>[2x]MTVPIAIIGTGIAGLSAAQALTSAGHQVH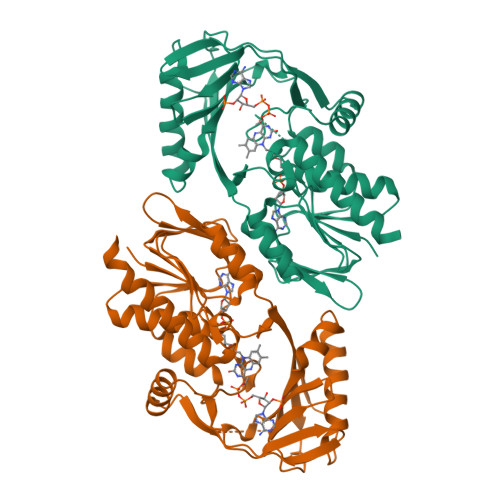LFDKSRGSGGRMSSKRSDAGSLDMGAQYFTARDRRFATAVKQWQAQGHVSEWTPLLYNFHGGRLSPSPDEQVRWVGEPGMSAITRAMRGDLPVSFSCRITDVFRGEQHWNLLDAESENHGPFSHVIIATPAPQATALLAAAPKLASVVAGVKMDPTWAVALAFETPLQTPMQGCFVQDSPLDWLARNRSKPGRDDTLDSWVLHATSQWSRQNLDASREQVIEHLHGAFAELIDCAMPAPVFSLAHRWLYARPAGSHEWGALSDADLGIYVCGDWCLSGRVEGAWLSGQEAARRLLEHLQLEHHHHHH>GAMNWTVDIPIDQLPSLPPLPTDLRTRLDAALAKPAAQQPTWPADQALAMRTVLESVPPVTVPSEIVRLQEQLAQVAKGEAFLLQGGDCAETFMDNTEPHIRGNVRALLQMAVVLTYGASMPVVKVARIAGQYAKPRSADIDALGLRSYRGDMINGFAPDAAAREHDPSRLVRAYANASAAMNLVRALTSSGLASLHLVHDWNREFVRTSPAGARYEALATEIDRGLRFMSACGVADRNLQTAEIYASHEALVLDYERAMLRLSDGDDGEPQLFDLSAHTVWIGERTRQIDGAHIAFAQVIANPVGVKLGPNMTPELAVEYVERLDPHNKPGRLTLVSRMGNHKVRDLLPPIVEK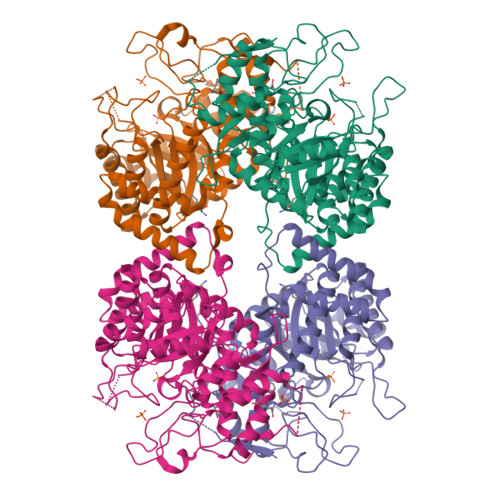VQATGHQVIWQCDPMHGNTHESSTGFKTRHFDRIVDEVQGFFEVHRALGTHPGGIHVEITGENVTECLGGAQDISETDLAGRYETACDPRLNTQQSLELAFLVAEMLRD[2x]>[2x]TG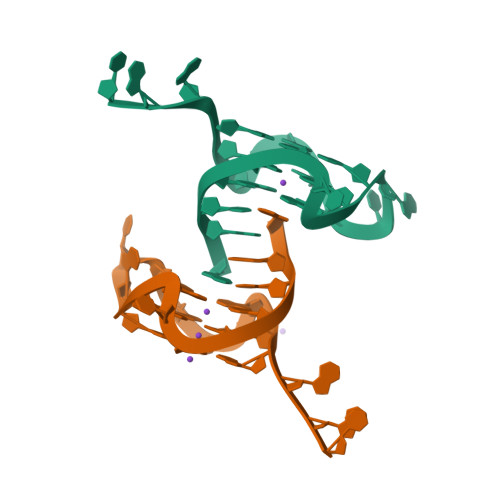AGGGTGGGTAGGGTGGGTAA>[2x]TDTTLPPDDSLDRIEPVDIEQEMQRSYIDYAMSVIVGRALPEVRDGLKPVHRRVLYAMFDSGFRPDRSHAKSARSVAETMGNYHPHGDASIYDSLVRMAQPWSLRYPLVDGQGNFGSPGNDPPAAMRFTEARLTPLAMEMLREIDEETVDFIPNYDGRVQEPTVLPSRFPNLLANGSGGIAVGMATNIPPHNLRELADAVFWALENHDADEEETLAAVMGRVKGPDFPTAGLIVGSQGTADAYKTGRGSIRMRGVVEVEEDSRGRTSLVITELPYQVNHDNFITSIAEQVRDGKLAGISNIEDQSSDRVGLRIVIEIKRDAVAKVVINNLYKHTQLQTSFGANMLAIVDGVPRTLRLDQLIRYYVDHQLDVIVRRTTYRLRKANERAHILRGLVKALDALDEVIALIRASETVDIARAGL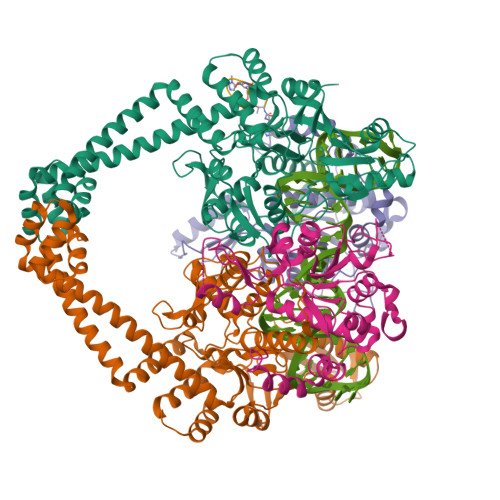IELLDIDEIQAQAILDMQLRRLAALERQRIIDDLAKIEAEIADLEDILAKPERQRGIVRDELAEIVDRHGDDRRTRIIAA;>[2x]ELVRRKSATDIGGLPGKLADCRSTDPRKSELYVVEGDSAGGSAKSGRDSMFQAILPLRGKIINVEKARIDRVLKNTEVQAIITALGTGIHDEFDIGKLRYHKIVLMADADVDGQHISTLLLTLLFRFMRPLIENGHVFLAQPPLYKLKWQRSDPEFAYSDRERDGLLEAGLKAGKKINKEDGIQRYKGLGEMDAKELWETTMDPSVRVLRQVTLDDAAAADELFSILMGEDVDARRSFITRNAKDVRFLDV;> XTRTXDSFGRSD> SNAGASCTYVWSDWNKCVCPMG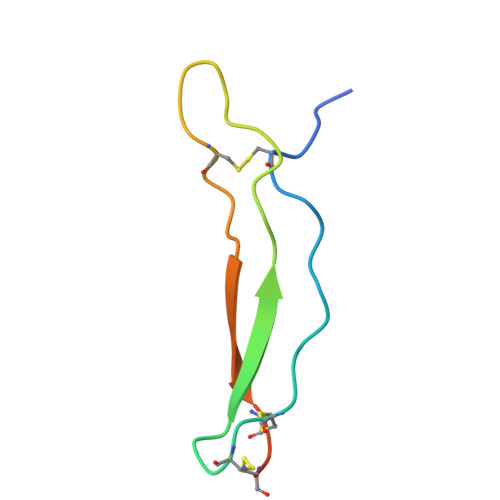YQARHAAVKFDYRNKPCDLPTFETKACSCGETNPVP>[2x]LTPEQIIAVDGAHLWHPYSSIGREAVSPVVAVAAHGAWLTLIRDGQPIEVLDAMSSWWTAIHGHGHPALDQALTTQLRVMNHVMFGGLTHEPAARLAKLLVDITPAGLDTVFFSDSGSVSVEVAAKMALQYWRGRGLPGKRRLMTWRGGYHGDTFLAMSICDPHGGMHSLWTDVLA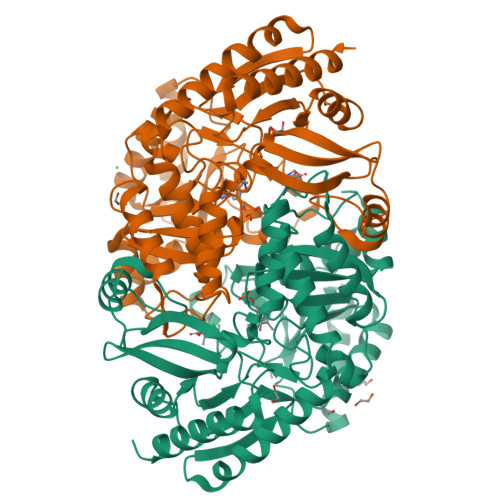AQVFAPQVPRDYDPAYSAAFEAQLAQHAGELAAVVVEPVVQGAGGMRFHDPRYLHDLRDICRRYEVLLIFDEIATGFGRTGALFAADHAGVSPDIMCVGKALTGGYLSLAATLCTADVAHTISAGAAGALMHGPTFMANPLACAVSVASVELLLGQDWRTRITELAAGLTAGLDTARALPAVTDVRVCGAIGVIECDRPVDLAVATPAALDRGVWLRPFRNLVYAMPPYICTPAEITQITSAMVEVARLVGSL We show that the orthologue identified in A. hydrophila (AhlABC) is a haemolytic tripartite α-PFT, requiring all three components for maximal lysis, and we present the structures of the soluble forms of monomeric AhlB and tetrameric AhlC and the decameric pore form of AhlB. AhlC provides the initial single leaflet insertion, assembly with AhlB then producing an oligomeric hydrophobic pore, and finally recruitment of AhlA produces a hydrophilic fully active AhlABC pore. Structural and sequence analysis suggests this method of pore assembly may well occur throughout the tripartite α-PFT family.

The structure of AhlB was determined to 2.9 Å in space group C2 (Form 1), using Se-Methionine SAD and subsequently the resolution was extended to 2.5 Å, using data from a crystal in space group C2221 (Form 2). In the AhlB pore one of each of the subunit conformations of AhlB pack together to form a dimer and five of these Type 1/Type 2 dimers assemble into the decameric oligomer. Within the oligomeric pore, AhlB adopts two subunit conformations, which vary at both the tail and head regions. In the Type 2 conformation residues from both hinges adopt helical conformations, forming sections of α3 and α4, whereas in the Type 1 conformation, the hinge 1 residues in α3 (K152–L160) remain in a loop, indicating that the Type 2 conformation is the fully extended form. Furthermore, in Type 1 the N-terminal helix (α1) is sandwiched between helices α4 and α5, whereas in the Type 2 conformation the first 15 residues of α1 are disordered, with the N-terminus of α1 packing against the C terminus of α5 in an end-to-end arrangement. Thus, the Type 1 conformation has a five-helix bundle at the tail, whereas the Type 2 conformation has a four-helix bundle at the tail. Each subunit of the pore is constructed from two extended α-helices (α3 and α4) that join the head of the pore to the five α-helices that fold into the pore tail. In this soluble to pore transition, changes in ɸ and ψ angles of up to 180o for the hinge residues and movements of up 94 Å result in both the β-tongue and α3a/α4a (D156-L186 and G225-Q246) unpacking and the secondary structure rearranging to form the two 140 Å extended helices (α3 and α4), constructing the head of the funnel and presenting this hydrophobic head to the membrane. The first 15 N-terminal residues of the Type 2 subunits point towards the centre of the oligomer where discontinuous electron density is observed, perhaps suggesting that these residues may form a plug in the entrance to the funnel resulting in an inactive pore, possibly explaining the lack of haemolytic activity of AhlB alone.

>[10x]MTNATTITMDQGMANQASQAMQIQTYCNSVKQQVPVDFSQFPNLKDNQTQINQGLDLAKGHADLYLNTIQPQIITNISNISNYFALQNAIPAVLPPGSTKAQWLRQLSVIKEQATEYQRLSSDTRLVIVNLNNNLITDSSNFQGIVVNLNSKVQGDNGVLAQLNGDIDKVNAAIDGAIAGIVAGGLLVIGGAFVTAIGAVADFVTAGTSTPVVIGGVAMMVAGAGGITAGAIVLHNSLGARQDLYQKRSSLNSEVLIATQIGNGYKGLQVQAQNAVTAATQMSNAWDSLTSDLGSLITDLDKGITSGDDIRQLWLTAADTTVKTVLTDVTTIKAQIAGVSPLQVPQTDTIANFVARLAALEHHHHHH>[18x]MFIQEPKKLIDTGEIGNASTGDILFDGGNKINSDFNAIYNAFGDQRKMAVANGTGADGQIIHATGYYQKHSITEYATPVKVGTRHDIDTSTVGVKV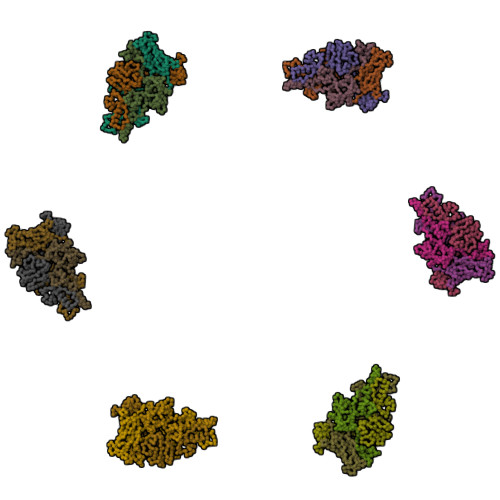IIERGELGDCVEFINSNGSISVTNPLTIQAIDSIKGVSGNLVVTSPYSKVTLRCISSDNSTSVWNYSIESMFGQKESPAEGTWNISTSGSVDIPLFHRTEYNMAKLLVTCQSVDGRKIKTAEINILVDTVNSEVISSEYAVMRVGNETEEDEIANIAFSIKENYVTATISSSTVGMRAAVKVIATQKIGVAQ>[26x]MPFAEDKTYKYICRNFSNFCNVDVVEILPYLPCLTARDQDRLRAT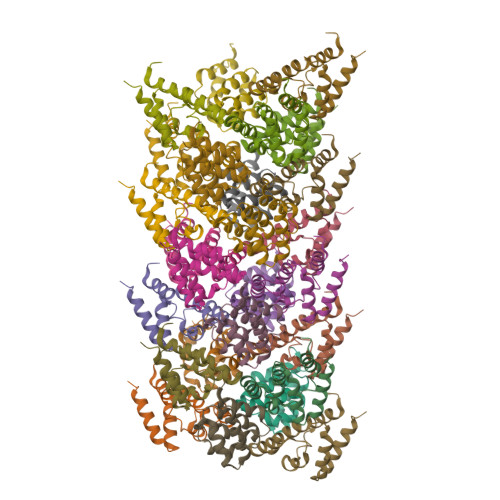CTLSGNRDTLWHLFNTLQRRPGWVEYFIAALRGCELVDLADEVASVYQSYQP> GAQNQDCAFFFPNQEGEQITRNCYTADGKLTNILVYRVDQAYEYPSGMEVVANYTFADAAGKTLNSGQMVARCSDGNFSMSMGDVATFPTALNMMNADVYMMGDLMNYPDAFSNPMNPGDDDEFDDGTLRLYQKGNKNNRAEISVFDREFVTT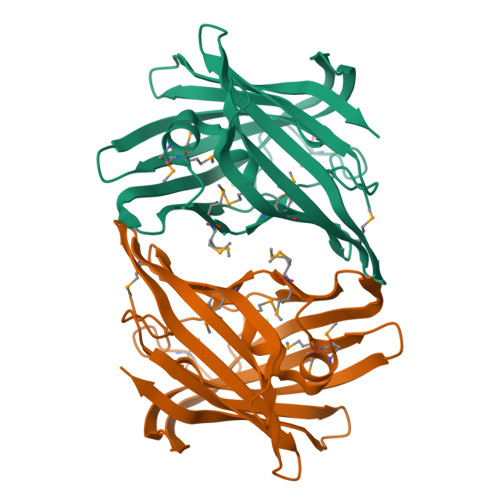ETVNTPAGAFYCTKVKYEMNIWTPKETIKGYGYEWYAPNIGIVRSEQYNNKKELQSYSVLERIKK Tpt1 is a fascinating enzyme that transfers an internal RNA 2′-monophosphate (2′-PO4) to NAD+ to form a 2′-OH RNA and ADP-ribose-1″,2″-cyclic phosphate. The Tpt1 mechanism comprises two chemical steps in which: (i) the RNA 2′-PO4 reacts with NAD+ to expel nicotinamide and form a 2′-phospho-ADP-ribosylated RNA intermediate; and (ii) transesterification of the ADP-ribose 2′′-OH to the RNA 2′-PO4 displaces the RNA 2′-OH and generates ADP-ribose-1″,2″-cyclic phosphate. We succeeded in growing crystals of Tpt1 from the mesothermophilic bacterium Clostridium thermocellum (Cth) using recombinant CthTpt1 produced in E. coli. Hexagonal CthTpt1 crystals were in space group P6122 and diffracted X-rays to 1.4 Å resolution. The refined Tpt1 structure (Rwork/Rfree 16.16/18.57) comprised a continuous polypeptide from Leu3 to Glu182, consisting of nine β strands, six α helices, and four 310 helices, organized into two distinct lobes spanning amino acids 1–85 and 86–182, respectively.

Here we close this gap by attaining a 1.4 Å crystal structure of Tpt1, providentially captured in a complex with ADP-ribose-1″-phosphate in the NAD+ site (generated during protein production in E. coli) and the pAp moiety of coenzyme A in the RNA site. This structure, which mimics the step 2 product complex of the Tpt1 reaction, yields keen insights into how Tpt1 recognizes a 2′-PO4 RNA splice junction. The 1.4 Å electron density map revealed two non-protein ligands bound to Tpt1 that were acquired during production of the recombinant protein in E. coli. The molecule associated with the C-terminal lobe was unambiguously modeled as ADP-ribose-1″-phosphate based on the electron density and the anomalous difference peaks overlying the three phosphorus atoms. The molecule associated with the N-terminal lobe was convincingly modeled as coenzyme A (CoA) based on: (i) the density of the terminal ppAp moiety in the Tpt1 active site and the anomalous difference peaks overlying the phosphorus atoms of the terminal pAp moiety, (ii) the electron density flanking ppAp corresponding to the pantetheine moiety of CoA, and (iii) covalent attachment of the terminal CoA sulfur to Tpt1 via a disulfide bond to Cys46. The pAp terminus of CoA is a mimetic of the dephosphorylated RNA product of the canonical Tpt1 reaction pathway. We envision that: (i) an endogenous substrate dissociated from Tpt1 after transfer of its phosphate to NAD+ to form ADP-ribose-1″,2″-cyclic phosphate; (ii) the RNA product site was then fortuitously occupied by the pAp moiety of CoA, present in the E. coli cytosol at 1.3 mM concentration; and (iii) CoA remained bound to Tpt1 during purification because it was covalently tethered to Cys46.

> MVLIDYSKLSKEVAYALRHAPWEYGLELDAEGWVDINQLLSSLHECEKWKKVSEHDLHVMIEKSDKKRYEISNGKIRALYGHSIPQRIIKEQKCPPEVLYHGTARRFVKSIKEKGLQPQGRQYVHLSADVETALQVGKRRDIKPVLLIVNALEAWSEGIKFYLGNDKVWLADAIPSKYIRFE>[6x]KLPAEFITRPHPSKDHGKETCTAYIHPNVLSSLEINPGSFCTVGKIGENGILVIARAGDEEVHPVNVITLSTTIRSVGNLILGDRLELKKAQVQPPYATKVTVGSLQGYNILECMEEKVIQKLLDDSGVIMPGMIFQNLKTKAGDESIDVVITDASDDSLPDVSQLDLNMDDMYGGLDNLFYLSPPFIFRKGSTHITFSKETQANRKYNLPEPLSYAAVGGLDKEIESLKSAIEIPLHQPTLFSSFGVSPPRGILLHGPPGTGKTMLLRVVANTSNAHVLTINGPSIVSKYLGETEAALRDIFNEARKYQPSIIFIDEIDSIAPNRANDDSGEVESRVVATLLTLMDGMGAAGKVVVIAATNRPNSVDPALRRPGRFDQEVEIGIPDVDARFDILTKQFSRMSSDRHVLDSEAIKYIASKTHGYVGADLTALCRESVMKTIQRGLGTDANIDKFSLKVTLKDVESAMVDIRPSAMREIFLEMPKVYWSDIGGQEELKTKMKEMI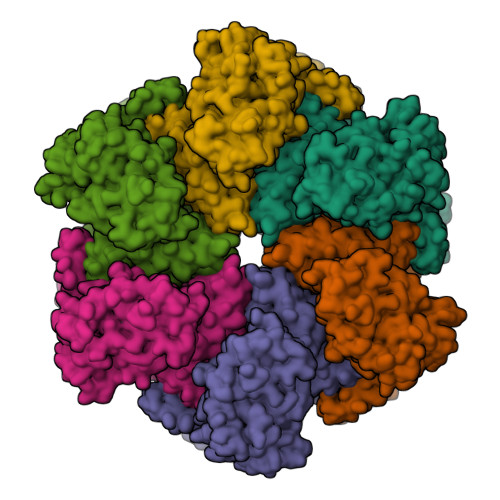QLPLEASETFARLGISAPKGVLLYGPPGCSKTLTAKALATESGINFLAVKGPEIFNKYVGESERAIREIFRKARSAAPSIIFFDEIDALSPDRDGSSTSAANHVLTSLLNEIDGVEELKGVVIVAATNRPDEIDAALLRPGRLDRHIYVGPPDVNARLEILKKCTKKFNTEESGVDLHELADRTEGYSGAEVVLLCQEAGLAAIMEDLDVAKVELRHFEKAFKGIARGITPEMLSYYEEFALRS Using soluble chitin derivatives as oligoglycosyl donor and oligosaccharides derived from chitin and β-1,3-glucan as acceptors, A. fumigatus Crh enzymes act as transglycosylases for formation of chitin–chitin and chitin–glucan crosslinks both in vitro and in vivo. AfCrh5 adopts the GH16 family β-jelly-roll fold composed of two stacked seven-stranded β-sheets with a convex and a concave face. AfCrh5 shares the general EXDXE active site motif present in most GH16 family enzymes in which the first glutamate, the middle aspartate and the last glutamate act as the catalytic nucleophile, the auxiliary residue, and the general acid/base, respectively. In AfCrh5, Glu119 and Glu123 are predicted to act as the nucleophile and the general acid/base, respectively.

The best of these was a chitin tetrasaccharide (NAG4) soak displaying diffraction to 2.8 Å. Initial electron density defined the positions of NAG4 and chitobiose (NAG2), which were located in the donor (−4 to −1) and acceptor (+1 to +2)-binding sites on the concave face, respectively. The −1 O6 hydroxyl interacts with Glu123, Ser109 and Trp207 side chains, and the −1 O1 hydroxyl interacts with Asp121. The sugar moiety in the −2 subsite establishes two types of interactions: a CH–π interaction between the sugar moiety and Trp207, and hydrogen bonds between Arg203 and the carbonyl group and between water molecules and the O3 hydroxyl/amide group. The sugar moieties located at −3 and −4 subsites do not establish any direct interactions with the enzyme and only the −3 carbonyl group is engaged to a water molecule by a hydrogen bond interaction. The +1 sugar moiety is tethered by Trp221, Asn135 and Glu123. There are CH–π interactions between the sugar moiety and Trp221, and hydrogen bonds between the O3 hydroxyl with Asn135, and the O4 hydroxyl with Glu123. Finally, the +2 sugar moiety establishes a CH–π interaction with Tyr145 and a hydrogen bond between the O3 hydroxyl and Thr218. As suggested by the crystal structure, these hydrolysis products may still bind the +1/+2 acceptor subsites, thus excluding potential nearby water molecules that would lead to premature hydrolysis of the covalent glycosyl–enzyme intermediate.

>WSKCNPLEKTCPPNKGLAASTYTADFTSASALDQWEVTAGKVPVGPQGAEFTVAKQGDAPTIDTDFYFFFGKAEVVMKAAPGTGVVSSIVLESDDLDEVDWEVLGGDTTQVQTNYFGKGDTTTYDRGTYVPVATPQETFHTYTIDWTKDAVTWSIDGAVVRTLTYNDAKGGTRFPQTPMRLRLGSWAGGDPSNPKGTIEWAGGLTDYSAGPYTMYVKSVRIENANPAESYTYSDNSGSWQSIKFD[2x]>LDNGLARTPTMGWLHWERFMCNLDCQEEPDSCISEKLFMEMAELMVSEGWKDAGYEYLCIDDCWMAPQRDSEGRLQADPQRFPHGIRQLANYVHSKGLKLGIYADVGNKTCAGFPGSFGYYDIDAQTFADWGVDLLKFAGCYCDSLENLADGYKHMSLALNRTGRSIVYSCEWPLYMWPFQKPNYTEIRQYCNHWRNFADIDDSWKSIKSILDWTSFNQERIVDVAGPGGWNDPDMLVIGNFGLSWNQQVTQMALWAIMAAPLFMSNDLRHISPQAKALLQDKDVIAINQDPLGKQGYQLRQGDNFEVWERPLSGLAWAVAMINRQEIGGPRSYTIAVASLGKGVACNPACFITQLLPVKRKLGFYEWTS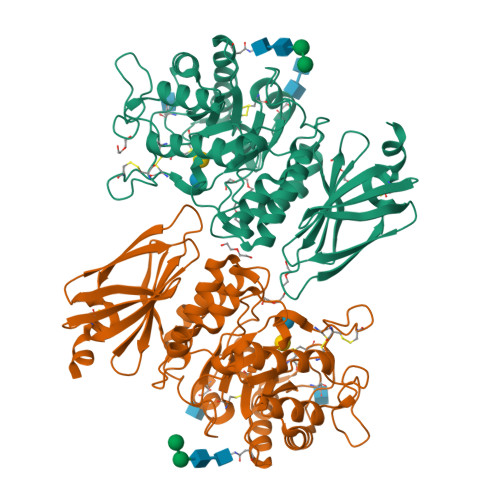RLRSHINPTGTVLLQLENTMQMSLKDLLHHHHHH[2x]> MDEKTKKAEEMAL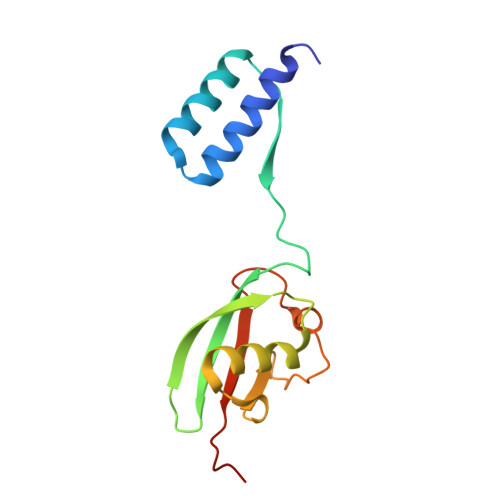SLARAVAGGDEQAAIKYATWLAEQRVPLRVQVKPEVSPTQDIRLCVSVEDAYMHTVTIWLTVRPDMTVASLKDMVFLDYGFPPSLQQWVVGQRLARDQETLHSHGIRRNGDGAYLYLLSARNTSLNP> PISPIETVPVKLKPGMDGPKVKQWPLTEEKIKALVEICTEMEKEGKISKIGPENPYNTPVFAIKKKDSTKWRKLVDFRELNKRTQDFWEVQLGIPHPAGLKKKKSVTV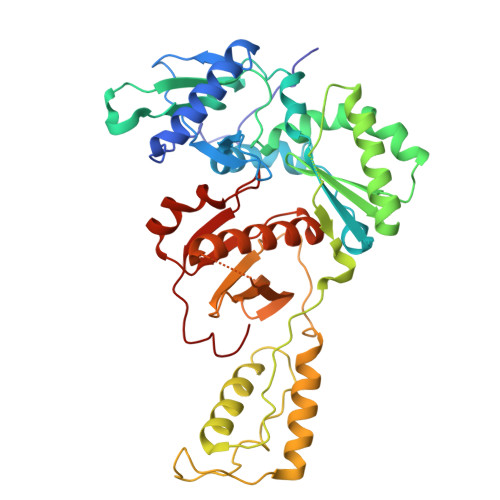LDVGDAYFSVPLDEDFRKYTAFTIPSINNETPGIRYQYNVLPQGWKGSPAIFQSSMTKILEPFKKQNPDIVIYQYMDDLYVGSDLEIGQHRTKIEELRQHLLRWGLTTPDKKHQKEPPFLWMGYELHPDKWTVQPIVLPEKDSWTVNDIQKLVGKLNWASQIYPGIKVRQLCKLLRGTKALTEVIPLTEEAELELAENREILKEPVHGVYYDPSKDLIAEIQKQGQGQWTYQIYQEPFKNLKTGKYARMRGAHTNDVKQLTEAVQKITTESIVIWGKTPKFKLPIQKETWETWWTEYWQATWIPEWEFVNTPPLVKLWY> SNASYETSQHNLDAVEAVLSRLQKQTGEMAAYMVPVGYRALCVSQRESMQALRCSFVQGQSQPLLRGASSKVMLAYMPAARCEKILRYFGEDPTLDKWQSEFEKI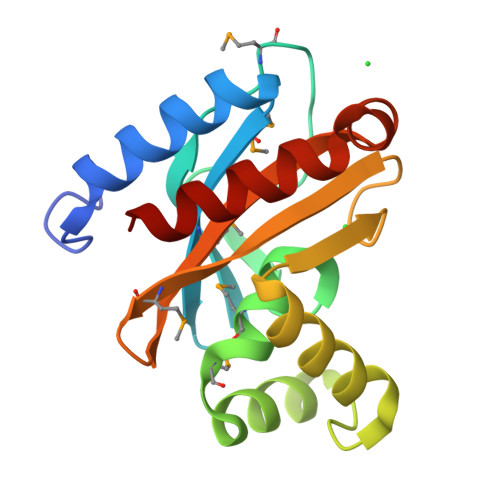RRHGYAVSTSEIDPGVSGISAPVMKGSKLIGAISVMAPAHRVESNKQRIILHVLQAARAL> MKKVVTVCPYCASGCKINLVVDNGKIVRAEAAQGKTNQGTLCLKGYYG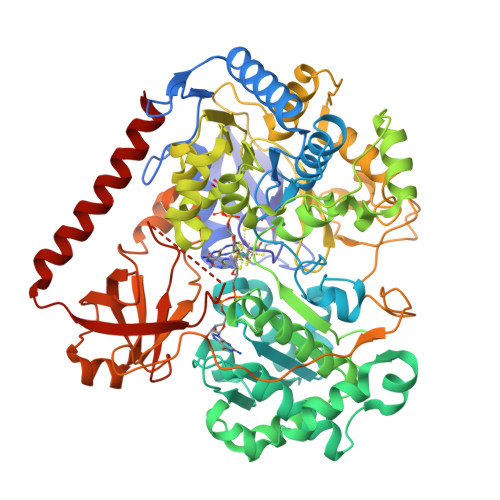WDFINDTQILTPRLKTPMIRRQRGGKLEPVSWDEALNYVAERLSAIKEKYGPDAIQTTGSSRGTGNETNYVMQKFARAVIGTNNVDCCARVUHGPSVAGLHQSVGNGAMSNAINEIDNTDLVFVFGYNPADSHPIVANHVINAKRNGAKIIVCDPRKIETARIADMHIALKNGSNIALLNAMGHVIIEENLYDKAFVASRTEGFEEYRKIVEGYTPESVEDITGVSASEIRQAARMYAQAKSAAILWGMGVTQFYQGVETVRSLTSLAMLTGNLGKPHAGVNPVRGQNNVQGACDMGALPDTYPGYQYVKDPANREKFAKAWGVESLPAHTGYRISELPHRAAHGEVRAAYIMGEDPLQTDAELSAVRKAFEDLELVIVQDIFMTKTASAADVILPSTSWGEHEGVFTAADRGFQRFFKAVEPKWDLKTDWQIISEIATRMGYPMHYNNTQEIWDELRHLCPDFYGATYEKMGELGFIQWPCRDTSDADQGTSYLFKEKFDTPNGLAQFFTCDWVAPIDKLTDEYPMVLSTVREVGHYSCRSMTGNCAALAALADEPGYAQINTEDAKRLGIEDEALVWVHSRKGKIITRAQVSDRPNKGAIYMTYQWWIGACNELVTENLSPITKTPEYKYCAVRVEPIADQRAAEQYVIDEYNKLKTRLREAALA>MSDEVSSSTDVVSRKRRRHDEGGKALEDIAVHGASEGDGSAPGGSVWQTTDYIALSMVVYRTAIKLRNFVNIRGLTPTEMIVIPWNVMRFYCEYNTGTYGLSGNVHHKNYSMLLACKAHRPTKVGYTLSNLILTSDELVSTGGTLGTTTTFNTSPYMIHSIDDQQCLSKVYPKTDTVWPVSSMRELDYVASTVSGDNAIIPSTIFNKNRYWKQGDDALHFSHDLDLGFWFGSDYGNAYVPQNNDSMNAVGTIPTSKHINVRGVNNRGMAGHYLSFPPIRTNDGQFKLNAQFTLETEIEFEFRLWEQGVQGINSVHTNLNPANDSLWIQSYGSLVS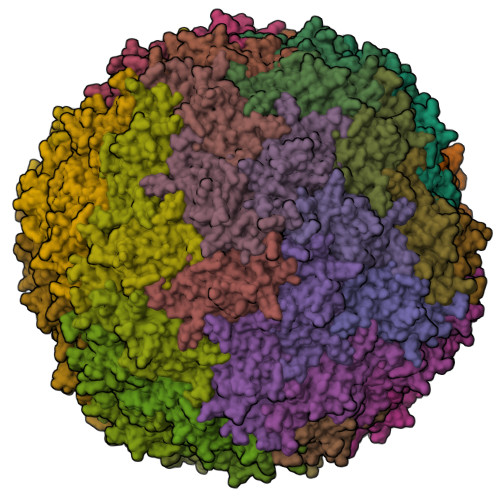ITESKINNIQFGPTCPRVDARNKGGKMSMLFDHH[60x]> MSFIKSLENRRTIYALGRNVQDEEKVIETIKEAVRFSPTAFNSQTGRLLILTGDAQDKLWDEIVAPELKAAMEAQGVPESAWDNTRAKLDGFKAAFGTILFFEDQAVVKNLQEQFALYADNFPVWSEQGSGIISVNVWTALAELGLGANLQHYNPLIDEAVAKEWNLPESWKL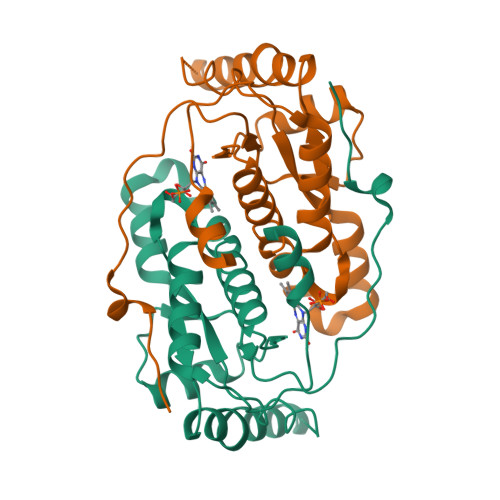RGQLVFGSIEAPAGEKTFMDDADRFIVAK> MANKRMKVKHDDHYELIVDGRVYYICIVCKRSYVCL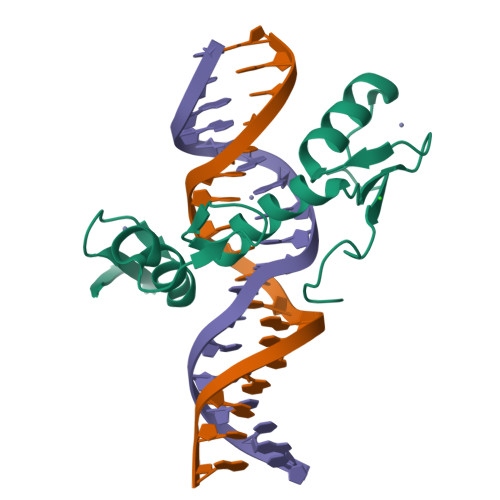TSLRRHFNIHSWEKKYPCRYCEKVFPLAQYRTKHEIHHTGERRYQCLACGKSFINYQFMSSHIKSVHSQDPSGDSKLYRLHPCRSLQIRQYAYLSDRS>[2x]MLHKKTLLFAALSAALWGGATQAADAAVVASLKPVGFIASAIADGVTETEVLLPDGASEHDYSLRPSDVKRLQNADLVVWVGPEMEAFMQKPVSKLPGAKQVTIAQLEDVKPLLMKSIHGDDDDHDHAEKSDEDHHHGDFNMHLWLSPEIARATAVAIHGKLVELMPQSRAKL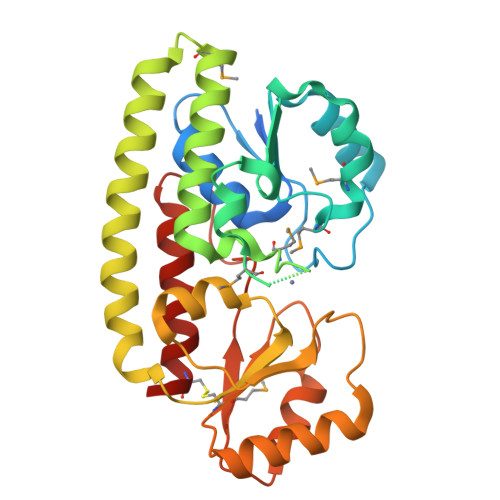DANLKDFEAQLASTETQVGNELAPLKGKGYFVFHDAYGYFEKQFGLTPLGHFTVNPEIQPGAQRLHEIRTQLVEQKATCVFAEPQFRPAVVESVARGTSVRMGTLDPLGTNIKLGKTSYSEFLSQLANQYASCLKGD QUINACRINE | C23 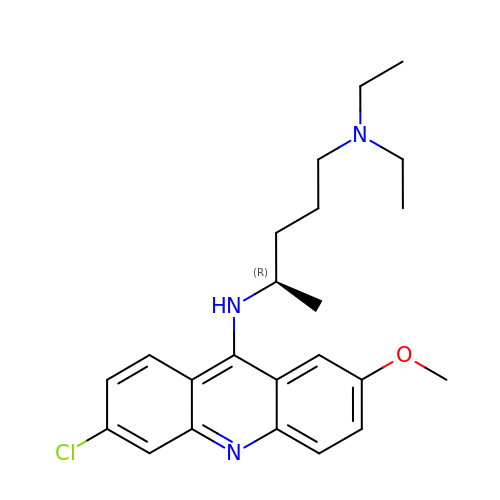H30 Cl N3 O | GPKJTRJOBQGKQK-MRXNPFEDSA-N3-methoxy-4-{[(6aR)-5-methyl-6-oxo-6,6a,7,8,9,10-hexahydro-5H-dipyrido[1,2-a:3',2'-e]pyrazin-2-yl]amino}-N-(1-methylpiperidin-4-yl)benzamide 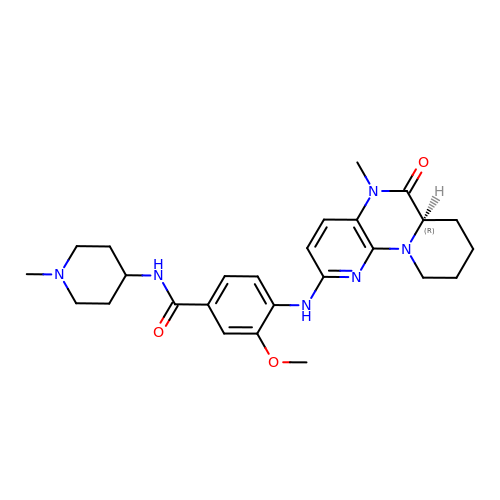| C26 H34 N6 O3 | AVGGLPRMVXANOV-OAQYLSRUSA-N> ADPHHHHHHENLYFQGQKLDDVDPLVTTNFGKIRGIKKELNNEILGPVIQFLGVPYAAPPTGEHRFQPPEPPSPWSDIRNATQFAPVCPQNIIDGRLPEVMLPVWFTNNLDVVSSYVQDQSEDCLYLNIYVPTEDDIRDSGGPKPVMVYIHGGSYMEGTGNLYDGSVLASYGNVIVITVNYRLGVLGFLSTGDQAAKGNYGLLDLIQALRWTSENIGFFGGDPLRITVFGSGAGGSCVNLLTLSHYSEGLFQRAIAQSGTALSSWAVSFQPAKYARILATKVGCQVSDTVELVECLQKKPYKELVDQDVQPARYHIAFGPVIDGDVIPDDPQILMEQGEFLNYDIMLGVNQGEGLKFVENIVDSDDGVSASDFDFAVSNFVDNLYGYPEGKDVLRETIKFMYTDWADRHNPETRRKTLLAL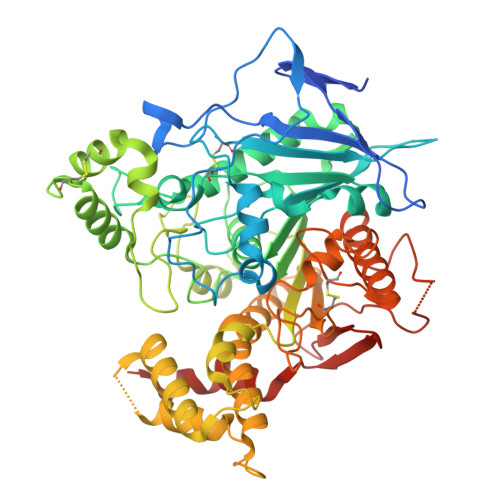FTDHQWVAPAVATADLHSNFGSPTYFYAFYHHCQTDQVPAWADAAHGDEVPYVLGIPMIGPTELFPCNFSKNDVMLSAVVMTYWTNFAKTGDPNQPVPQDTKFIHTKPNRFEEVAWTRYSQKDQLYLHIGLKPRVKEHYRANKVNLWLELVPHLHN> PRLSYPTFF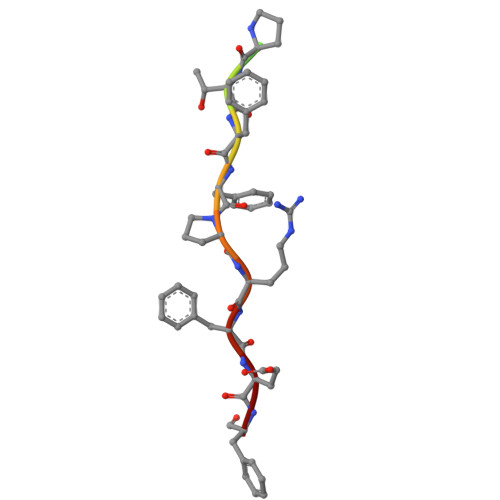PRFEF>GHMAAACRSVKGLVAVITGGASGLGLATAERLVGQGASAVLLDLPNSGGEAQAKKLGNNCVFAPADVTSEKDVQTALALAKGKFGRVDVAVNCAGIAVASKTYNLKKGQTHTLEDFQRVLDVNLMGTFNVIRLVAGEMGQNEPDQGGQRGVIINTASVAAFEGQVGQA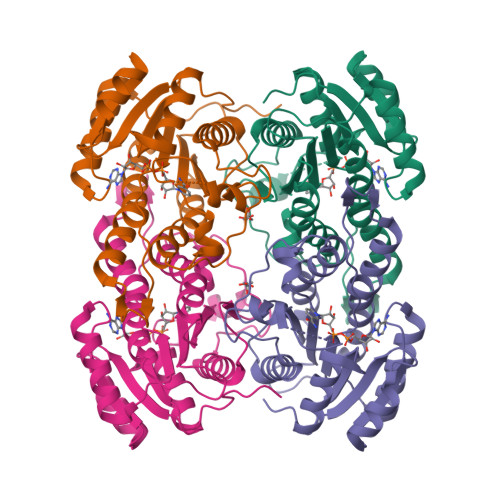AYSASKGGIVGMTLPIARDLAPIGIRVMTIAPGLFGTPLLTSLPEKVCNFLASQVPFPSRLGDPAEYAHLVQAIIENPFLNGEVIRLDGAIRMQPGS[2x]> TYNNSNPF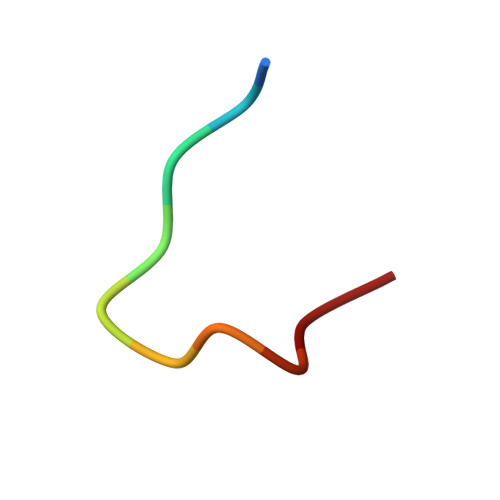MT> MRSTALRLYKMPKNMGVAPRFDVWNESYEPWQHMKRMGRLVGTGFYIPPEWYNHFRMFPPINHNFQQEKTLNPRNESEPTQDDTGSLSQERAALRDELARKSRLLASEGMRYYNIFWVRKPLDRMEKEYYELKRKGIAHSEAIKKVLEGFYKELAVKKRVAAVQAEEAKLSGRFITMREATVVLNVLAQLHREQLTPHQVTLLAREQHQATEKASGLTATVSRVSAPAAGIDADSTASKESGSDEALSADSLANML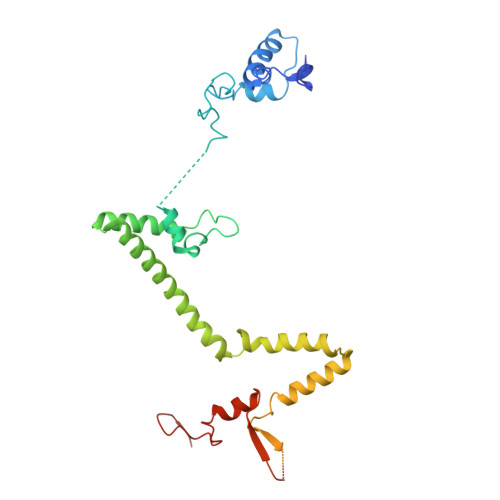EDDHASGAGTQYQVEVKHSARDSVRQLHEKSTDDTGSPDWYTGASPVYNGAA> MGSRLDKSKVINSALELLNEVGIEGLTTRKLAQKLGVEQPTLYWHVKNKRALLDAMAIEMLDRHATHYCPLEGESWQDFLRNNAKSMRCALLSHRDGAKVCLGTGFTEQQYETAENSLAFLCQQGFSL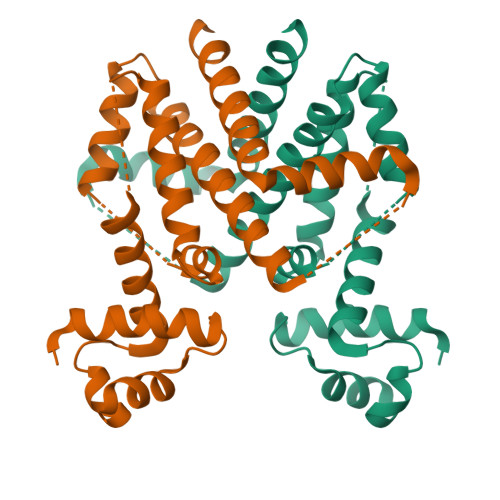EHAMYAMQAAGIYTLGCVLLDQELQVAKEERETPTTDSMPPLVRQALELKDHQGAEPAFLFGLELIICGLEKQLKCESGS> MQTLKELIASNPDDLTTELKRAFRPLTPHIAIDGNELDALTILVNLTDKTDDQKDLLDRAKCKQKLRDEKWWASCINCVNYRQSHNPKFPDIRSEGVIRTQALGELPSFLLSSSKIPPYHWSYSHDSKYVNKSAFLTNEFCWDGEISCLGELLKDADHPLWNTLKKLGCSQKTCKAMAKQLADITLTTINVTLAPNYLTQISLPDSDTSYISLSPVASLSMQSHFHQRLQDENRHSAITRFSRTTNMGVTAMTCGGAFRMLKSGAKFSSPPHHRLNSKRSWLTSEHVQSLKQYQRLNKSLIPENSRIALRRKYKIELQNMVRSWFAMQDHTLDSNILIQHLNHDLSYLGATKRFAYDPAMTKLFTELLKRELSNSINNGEQHTNGSFLVLPNIRVCGATALSSPVTVGIPSLTAFFGFVHAFERNINRTTSSFRVESFAICVHQLHVEKRGLTAEFVEKGDGTISAPATRDDWQCDVVFSLILNTNFAQHIDQDTLVTSLPKRLARGSAKIAIDDFKHINSFSTLETAIESLPIEAGRWLSLYAQSNNNLSDLLAAMTEDHQLMASCVGYHLLEEPKDKPNSLRGYKHAIAECIIGLINSITFSSETDPNTIFWSLKNYQNYLVVQPRSINDETTDKSSL;>MKLPTNLAYERSIDPSDVCFFVVWPDDRKTPLTYNSRTLLGQMEAASLAYDVSGQPIKSATAEALAQGNPHQVDFCHVPYGASHIECSFSVSFSSELRQPYKCNSSKVKQTLVQLVELYETKIGWTELATRYLMNICNGKWLWKNTRKAYCWNIVLTPWPWNGEKVGFEDIRTNYTSRQDFKNNKNWSAIVEMIKTAFSSTDGLAIFEVRATLHLPTNAMVRPSQVFTEKESGSKSKSKTQNSRVFQSTTIDGERSPILGAFKTGAAIATIDDWYPEATEPLRVGRFGVHREDVTCYRHPSTGKDFFSILQQAEHYIEVLSANKTPAQETINDMHFLMANLIKGGMFQHKGD[6x];> MKWYYKTITFLPELCNNESLAAKCLRVLHGFNYQYETRNIGVSFPLWCDATVGKKISFVSKNKIELDLLLKQHYFVQMEQLQYFHISNTVLVPEDCTYVSFRRCQSIDKLTAAGLARKIRRLEKRALSRGEQFDPSSFAQKEHTAIAHYHSLGESSKQTNRNFRLNIRMLSEQPREGNSIFSSYGLSNSENSFQPVPLI;>[2x]MFLQRPKPYSDESLESFFIRVANKNGYGDVHRFLEATKRFLQDIDHNGYQTFPTDITRINPYSAKNSSSARTASFLKLAQLTFNEPPELLGLAINRTNMKYSPSTSAVVRGAEVFPRSLLRTHSIPCCPLCLRENGYASYLWHFQGYEYCHSHNVPLITTCSCGKEFDYRVSGLKGICCKCKEPITLTSRENGHEAACTVSNWLAGHESKPLPNLPKSYRWG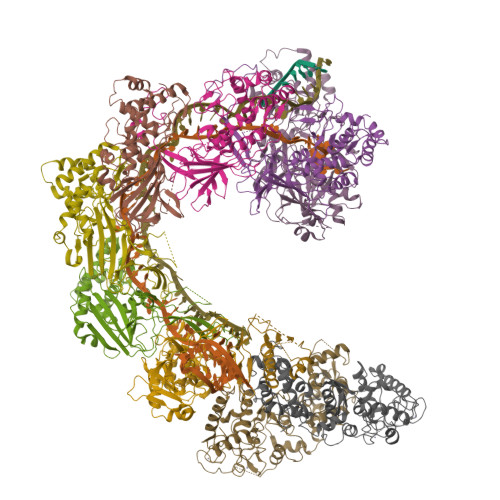LVHWWMGIKDSEFDHFSFVQFFSNWPRSFHSIIEDEVEFNLEHAVVSTSELRLKDLLGRLFFGSIRLPERNLQHNIILGELLCYLENRLWQDKGLIANLKMNALEATVMLNCSLDQIASMVEQRILKPNRKSKPNSPLDVTDYLFHFGDIFCLWLAEFQSDEFNRSFYVSRW>NENNTVVAETKTSTASETSEPKQVISSKQQLASLYLQAKQSLFKQRALSATMYGLSQKDIGQVISSDMEFYSPENEKQLRAELLSISNTIAGIKLDDADITTKNNQQVMAGLTRYFAGEPNFNIGYIDTWMGLSPFIVNQINGPLIDIPRVMQNDQPITTEKEALDYIVRLGQFDKLAATIIEKQTADAAQNWLPSKVTLQGAIKYLKGFTSGSAEQHPFVNVFREKIEKVDSLTTEQKQSLITQVIAKVSQVVYPAYQSVEKASEQLLSEARSESGIWAQPKGSVYYQDAIKQLGDSELSPTQIHQIGLDEVARISGVMNEILLAQGYTKGTVGERMVALNEEPRFLYEDSIAGREELLSDINGYITEVTAKMAPVFRTTPSYQVEVKSFPVEVQDGAPGGQYTSPAVDGSKPGIYWINLRDMKANPKFGLKTLTYHEANPGHHWQIALNLDQAELPFLRRIAPYNAYTEGWALYSEQVAYELGMYENDPFGDLGRLQAELFRAVRLVVDTGLHDKRWTREQAISYMSEQTGTAESDVVAEIERYM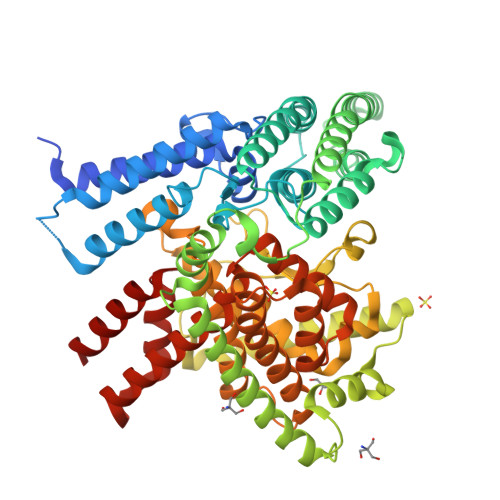AWPGQALGYKLGMLKILSLREQAKARLGDKFDLAEFHDVVLLNGAVPMAVLSRNVNHWLDNK[3x]>MSLGNASMTKTDIATRVHNHTWKLDPIVRSLIDTDFYKLLMLQMIWKLYPEVDATFSLINRTKTVRLAEEIDEMELREQLDHARTLRLSKKENIWLAGNTFYGRSQIFEPEFLSWLSSYQLPEYELFKRDGQYELNFHGRWMDTTLWEIPALSIINELRSRSAMRSLGYFTLDVLYARAKAKMWEKVERLRELPGLRISDFGTRRRHSFLWQRWCVEALKEGIGPAFTGTSNVLLAMDSDLEAVGTNAHELPMVVAALAQTNEELAAAPYQVLKDWNRLYGG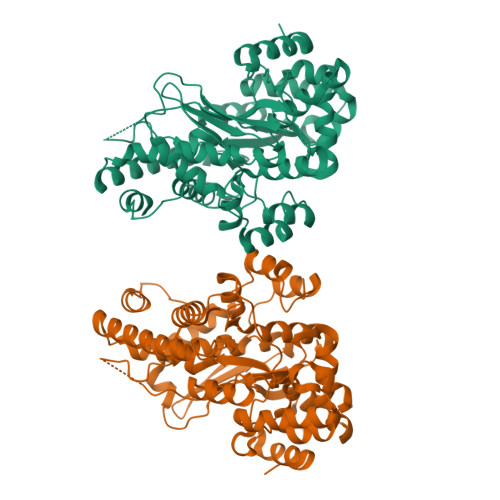NLLIVLPDAFGTAAFLRNAPEWVADWTGFRPDSAPPIEGGEKIIEWWRKMGRDPRTKMLIFSDGLDVDAIVDTYRHFEGRVRMSFGWGTNLTNDFAGCAPKTIASLKPISIVCKVSDANGRPAVKLSDNPQKATGDPAEVERYLKFFGEEDHKEQKVLVEGHHHHHH[2x]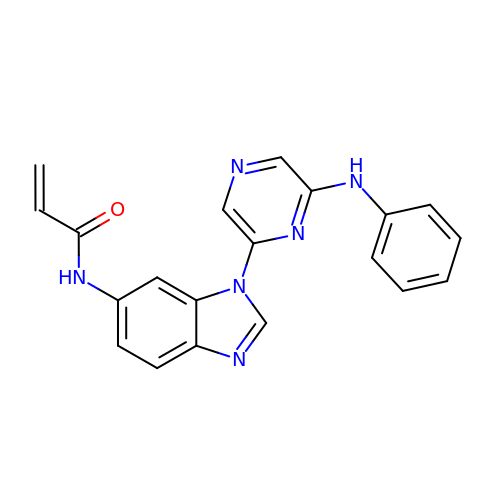N-{1-[6-(phenylamino)pyrazin-2-yl]-1H-benzimidazol-6-yl}prop-2-enamide | C20 H16 N6 O | CVFYLUGNOLKEFO-UHFFFAOYSA-N>GAMGSMATRIAILGAGPSGMAQLRAFQSAQEKGAEIPELVCFEKQADWGGQWNYTWRTGLDENGEPVHSSMYRYLWSDGPKECLEFADYTFDEHFGKPIASYPPREVLWDYIKGRVEKAGVRKYIRFNTAVRHVEFNEDSQTFTVTVQDHTTDTIYSAAFDYVVCCTGHFSTPYVPEFEGFEKFGGRILHAHDFRDALEFKDKTVLLVGSSYSAEDIGSQCYKYGAKKLISCYRTAPMGYKWPENWDERPNLVRVDTENAYFADGSSEKVDAIILCTGYIHHFPFLNDDLRLVTNNRLWPLNLYK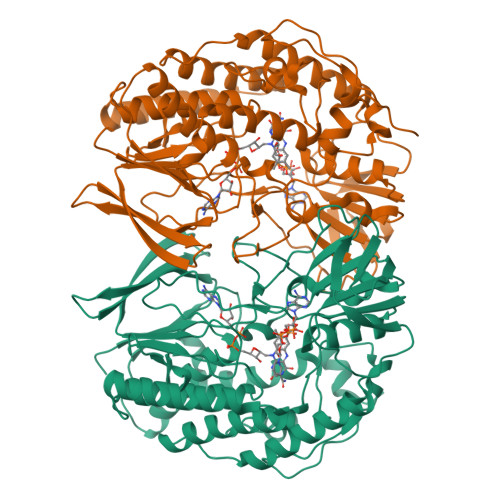GVVWEDNPKFFYIGMQDQWYSFNMFDAQAWYARDVIMGRLPLPSKEEMKADSMAWREKELTLVTAEEMYTYQGDYIQNLIDMTDYPSFDIPATNKTFLEWKHHKKENIMTFRDHSYRSLMTGTMAPKHHTPWIDALDDSLEAYLSDKSEIPVAKEA[4x]> MKPRIALFSCLMSLLSVPAHAALDPAQPLAEAPPYSLFEAWAKPVQPFAIWPGVWYVGTENLS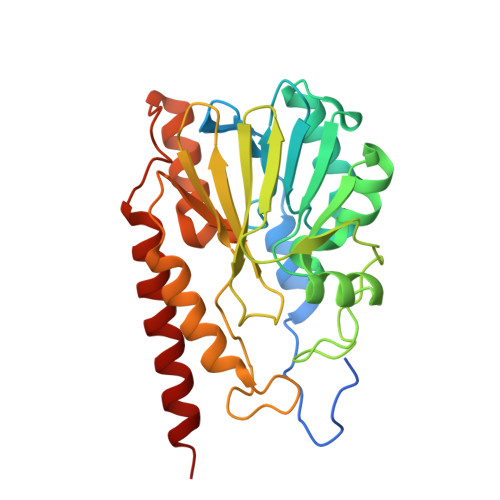SVLLTTPQGHILIDAGLDASAPQIRRNIEALGFRMADIRYIANSHARLDQAGGIARLKAWSGARVIASHANAEQMARGGKEDFALGDALPFPPVTVDMEAQDGQQWHLGGVTLAAIFTPGHLPGATSWKVTLADGKTLIYADSLATPGYPLINNRNYPTLVEDIRRSFARLEAQQVDIFLANKGERFGLMDKMARKARGENNAFIDKAGLARYVAQSRAAFEKQLAAQRAQP>GAMGRILFLTTFMSKGNKVVRYLESLHHEVVICQEKVHAQSANLQEIDWIVSYAYGYILDKEIVSRFRGRIINLHPSLLPWNKGRDPVFWSVWDETPKGVTIHLIDEHVDTGDILVQEEIAFADEDTLLDCYNKANQAIEELFIREWENIVHGRIAPYRQTAGGTLHFKADRDFYKNLNMTTVRELLALKRLCAEPKRGEKPIDKTFHQLFEQQVEMTPDHVAVVDRGQSLTYKQLNERANQLAHHLRGKGVKPDDQVAIMLDKSLDMIVSILAVMKAGGAYVPIDPDYPGERIAYMLADSSAAILLTNALHEEKANGACDIIDVHDPDSYSENTNNLPHVNRPDDLVYVMYTSGSTGLAKGVMIEHHNLVNFCEWYRPYFGVTPADKALVYSSFSFDGSALDIFTHLLAGAALHIVPSERKYDLDALNDYCNQEGITISYLPTGAAEQFMQMDNQSFRVVITGGDVLKKIERNGTYKLYNGYGPTECTIMVTMFEVDKPYANIPIGKPIDRTRILILDEALALQPIGVAGELFIVGEGLGRGYLNRPELTAEKFIVHPQTGERMYRTGDRARFLPDGNIEFLGRLDNLVKIRGYRIEPGEIEPFLMNHPLIELTTVLAKEQADGRKYLVGYYVAPEEIPHGELREWLGNDLPDYMIPTYFVHMKAFPLTANGKVDRRALPDVQADAELLGEDYVAPTDELEQQLAQVWSHVLGIPQMGIDDHFLERGGDSIKVMQLIHQLKNIGLSLRYDQLFTHPTIRQLKRLLTEQKQVSLEPLRELDEQAEYETSAVEKRMYIIQQQDVESIAYNVVYTINFPLTVDTEQIRVALEQLVLRHEGLRSTYHMRGDEIVKRIVPRAELSFVRQTGEEESVQSLLAEQIKPFDLAKAPLLRAGVIETADKKVLWFDSHHILLDGLSKSILARELQALLGQQVLSPVEKTYKSFARWQNEWFASDEYEQQIAYWKTLLQGELPAVQLPTKKRPPQLTFDGAIQMYRVNPEITRKLKATAAKHDLTLYMLMLTIVSIWLSKMNSDSNQVILGTVTDGRQHPDTRELLGMFVNTLPLLLSIDHEESFLHNLQQVKAKLLPALQNQYVPFDKILEAARVKREGNRHPLFDVMFMMQGAPETELESNMHHINAGISKFDLTLEVLERENGLNIVFEYNTHLFDEGMILRMVAQFEHLLLQAVHGLDQQVKRFELVTEDEKRDLFLRVNDTAKAYPNKLIMSMLEDWAAATPDKTALVFREQRVTYRELNERVNQLAHTLREKGVQPDDLVMLMAERSVEMMVAIFAVLKAGGAYLPIDPHSPAERIAYIFADSGAKLVLAQSPFVEKASMAEVVLDLNSASSYAADTSNPPLVN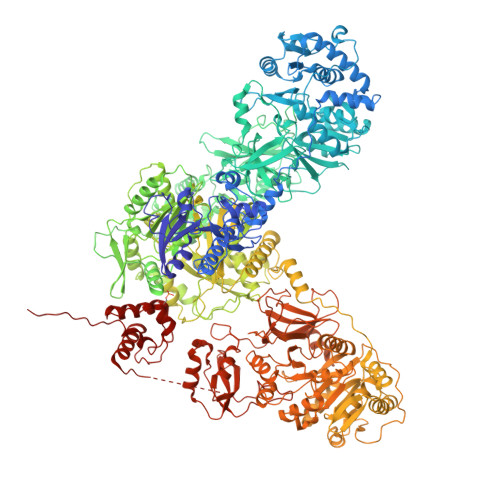QPGDLVYVMYTSGSTGKPKGVMIEHGALLNVLHGMQDEYPLLQDDAFLLKTTYIFDISVAEIFGWVPGRGKLVILEPEAEKNPKAIWQAVVGAGITHINFVPSMLIPFVEYLEGRTEANRLRYILACGEAMPDELVPKVYEVLPEVKLENIYGPTEATIYASRYSLAKGSQESPVPIGKPLPNYRMYIINRHGQLQPIGVPGELCIAGASLARGYLNNPALTEEKFTPHPLEKGERIYRTGDLARYREDGNIEYLGRMDHQVKIRGYRIELDEIRSKLIQEETIQDAVVVARNDQNGQAYLCAYLLSEQEWTVGQLRELLRRELPEYMIPAHFVLLKQFPLTANGKLDRKALPEPDGSVKAEAEYAAPRTELEATLAHIWGEVLGIERIGIRDNFFELGGDSIKGLQIASRLQRINWTMVINHLFLYPTIEQIAPFVTSEQVVIEAAAENLYFQ[2x]> MNSNLPAENLTIAVNMTKTLPTAVTHGFNSTNDPPSMSITRLFPALLECFGIVLCGYIAGRANVITSTQAKGLGNFVSRFALPALLFKNMVVLNFSNVDWSFLYSILIAKASVFFIVCVLTLLVASPDSRFSKAGLFPIFATQSNDFALGYPIVEALYQTTYPEYLQYIYLVAPISLMMLNPIGFIFCEIQKWKDTQNASQNKIKIVGLGLLRVLQNPIVFMVFIGIAFNFILDRKVPVYVENFLDGLGNSFSGSALFYLGLTMVGKIKRLKKSAFVVLILLITAKLLVLPLLCREMVELLDKGDSVVNHTSLSNYAFLYGVFPVAPGVAIFATQFNMEVEIITSGMVISTFVSAPIMYVSAWLLTFPTMDPKPLAYAIQNVSFDISIVSLISLIWSLAILLLSKKYKQLPHMLTTNLLIAQSIVCAGMMIWNFVKEKNFVGQILVFVLLYSSLYSTYLWTGLLAISLFLLKKRERVQIPVGIIIISGWGIPALLVGVLLITGKHNGDSIDSAFFYGKEQMITTAVTLFCSILIAGISLMCMNQTAQAGSYEGFDQSQSHKVVEPGNTAFEESPAPVNEPELFTSSIPETSCCSCSMGNGELHCPSIEPIANTSTSEPVIPSFEKNNHCVSRCNSQSCILAQEEEQYLQSGDQQLTRHVLLCLLLIIGLFAN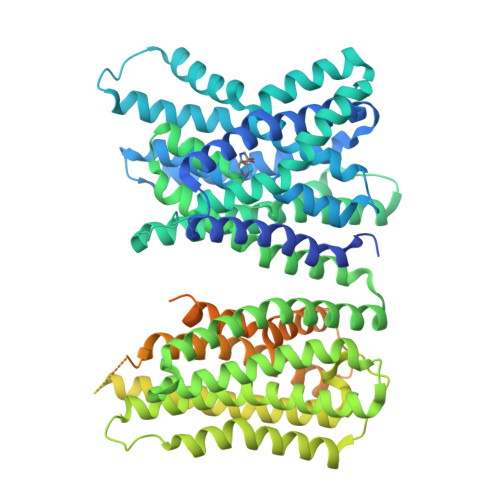LSSCLWWLFNQEPGRLYVELQFFCAVFNFGQGFISFGIFGLDKHLIILPFKRRLEFLWNNKDTAENRDSPVSEEIKMTCQQFIHYHRDLCIRNIVKERRCGAKTSAGTFCGCDLVSWLIEVGLASDRGEAVIYGDRLVQGGVIQHITNEYEFRDEYLFYRFLQKSPEQSPPAINANTLQQERYKEIEHSSPPSHSPKTGSGSDYKDDDDKDYKDDDDK> MTTTERPDLAWLDEVTMTQLERNPYEVYERLRAEAPLAFVPVLGSYVASTAEVCREVATS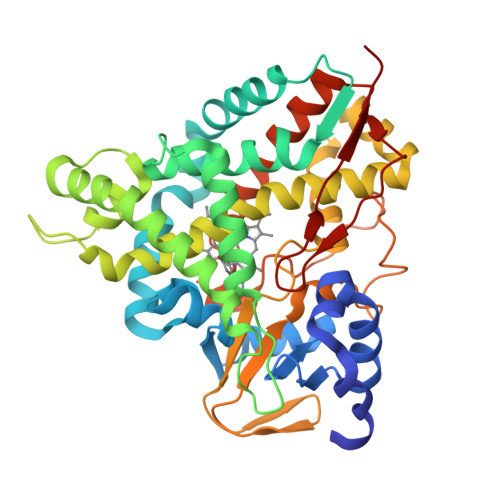PDFEAVITPAGGRTFGHPAIIGVNGDIHADLRSMVEPALQPAEVDRWIDDLVRPIARRYLERFENDGHAELVAQYCEPVSVRSLGDLLGLQEVDSDKLREWFAKLNRSSTNAAVDENGEFANPEGFAEGDQAKAEIRAVVDPLIDKWIEHPDDSAISHWLHDGMPPGQTRDREYIYPTIYVYLLGAMQEPGHGMASTLVGLFSRPEQLEEVVDDPTLIPRAIAEGLRWTSPIWSATARISTKPVTIAGVDLPAGTPVMLSYGSANHDTGKYEAPSQYDLHRPPLPHLAFGAGNHACAGIYFANHVMRIALEELFEAIPNLERDTREGVEFWGWGFRGPTSLHVTWEV> GGGRELPTLLSLLLEALSCPDSVVQLSTLSCLQPLLLEAPQIMSLHVDTLVTKFLNLSSSYSMAVRIAALQCMHA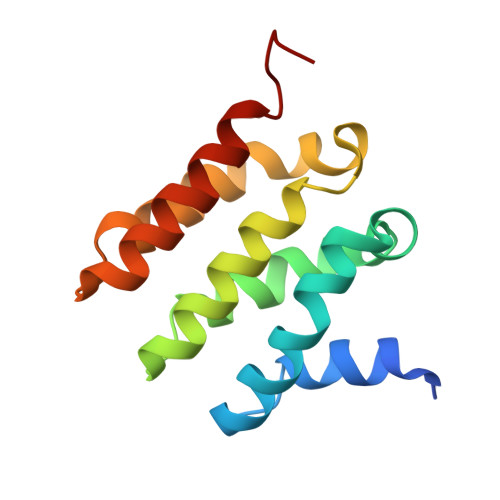LTRLPTSVLLPYKSQVIRALAKPLDDKKRLVRKEAVSARGEWFLLGSPGS>MGKVILVTGVSRGIGKSIVDVLFSLDKDTVVYGVARSEAPLKKLKEKYGDRFFYVVGDITEDSVLKQLVNAAVKGHGKIDSLVANAGVLEPVQNVNEIDVNAWKKLYDINFFSIVSLVGIALPELKKTNGNVVFVSSDACNMYFSSWGAYGSSKAALNHFAMTLANEERQVKAIAVAPGIVDTDMQVNIRENVGPSSMSAEQLKMFRGL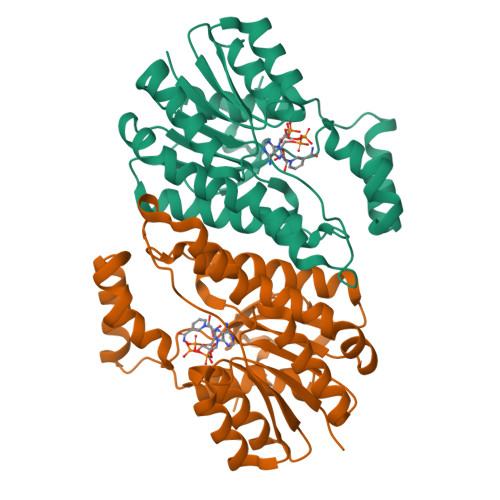KENNQLLDSSVPATVYAKLALHGIPDGVNGQYLSYNDPALADFMP[2x]>[2x]ACVFFCEDA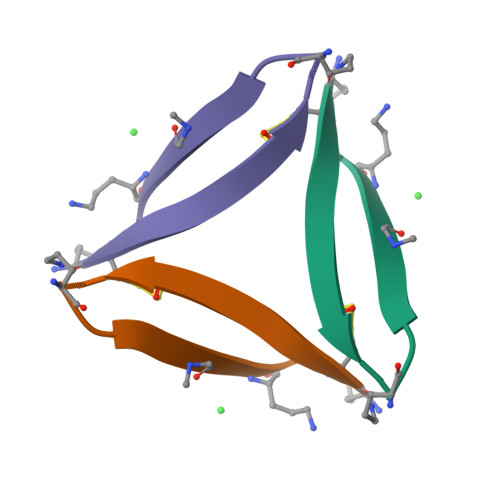AIIGLAV> MSNLLLLPIVIPLVTAIVLIFFPKHVFWQRVVSLAATVGLVVASGALLHRVHT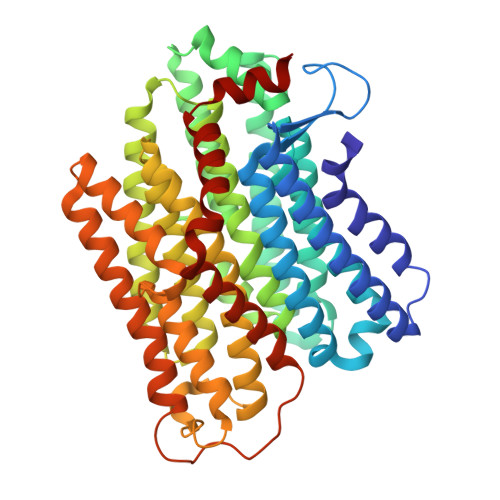DGIQTLNVGNWPAPFGITLVSDSLSALLVLTTSIIALACLVYSFYAIGHKRETFYYYSFFQFLIVGVNGAFTTGDLFNLFVFFEVMLMSSYVLLVLGGTKIQLRETIKYTLVNVISSALFVVAVAYLYAVTGTLNMAHLADRINALGSSPILTVIAVLFIIVFGLKGAIFPLYFWLPGAYYAPPTPVLALFGGLLTKVGVYSILRTFTLLFTHDAAYTHTLLAWLALGTIIIGVIGAVAYNDMRYIVIYNIIAAVGVMIFGISIMTPESVEGTIFYLLQDMVMKAMLFLFVGIIFSITRSNDIRSFSGLITSYPLLGWAFFIAALSLAGIPPLSGFIGKLLIVKASFDAQLIFEAIVILLSSLLVLYSVMKIFMNGFWGEKKGFEQKQVDGRLFPVLFLLVLSVAYGIGIEFVRPFVLDAVNVLVDPSMYIEAVLKE> MEAGITGTWYNQLGSTFIVTAGADGALTGTYVTARGNAESRYVLTGRYDSAPATDGSGTALGWTVAWKNNYRNAHSATT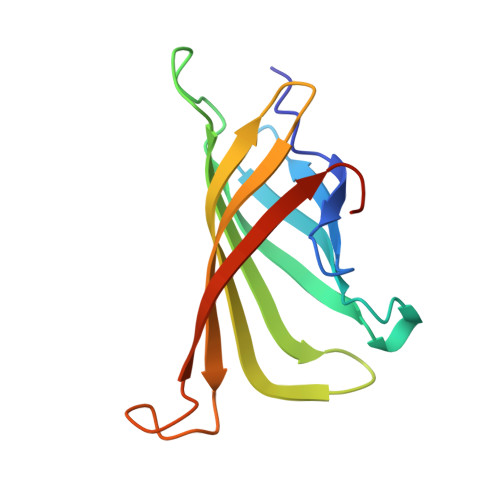WSGQYVGGAEARINTQWLLTSGTTEYNAFMSTLVGHDTFTKVKPSAAS>MASRGSHHHHHHGAAERALNDQLEFMRVLIDGTPNPIYVRDKEGRMLLCNDAYLDTFGVTADAVLGKTIPEANVVGDPALAREMHEFLLTRVAAEREPRFEDRDVTLHGRTRHVYQWTIPYGDSLGELKGIIGGWIDITER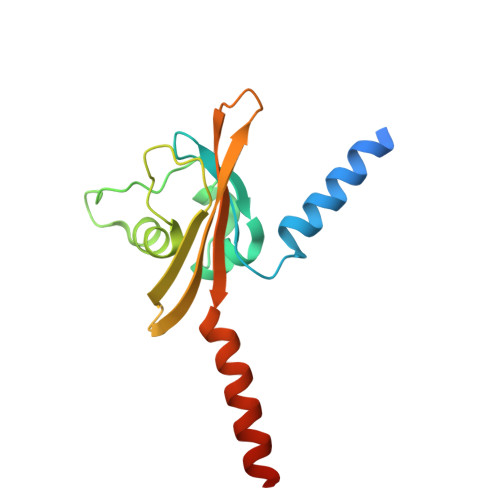AELLRKLHDLKESLDAANRAK[8x]>[2x]GAMNAQAEEFKKYLETNGIKPKQFHKKELIFNQWDPQEYCIFLYDGITKLTSISENGTIMNLQYYKGAFVIMSGFIDTETSVGYYNLEVISEQATAYVIKINELKELLSKNLTHFFYVFQTLQKQVSYSLAKFNDFSINGKLGSICGQLLILTYVYGKETPDGIKITLDNLTMQELGYSSGIAHSSAVSRIISKLKQEKVIVYKNSCFYVQNLDYLKRYAPKLDEWFYLACPATWGKLN

Expression of these L. monocytogenes virulence genes is controlled by positive regulatory factor A, PrfA. PrfA belongs to the cyclic AMP receptor protein-fumarate and nitrate reduction regulator (Crp-Fnr) family of bacterial transcription factors. Transcription factors of this family bind a wide range of ligands and are activated by allosteric communication between the ligand binding site and DNA-binding helix-turn-helix (HTH) motifs. Reduced glutathione (GSH), a low molecular weight thiol important for intracellular redox homeostasis, is thus far the only known allosteric activator of PrfA.

To verify and elucidate structural details of PrfA inhibition by IWP-2, we determined the crystal structure of the PrfA:IWP-2 complex at 2.0 Å resolution. The asymmetric unit of the PrfA:IWP-2 complex crystals contained one PrfA dimer composed of monomers A and B. Difference Fourier and Polder electron density maps unambiguously confirmed binding of IWP-2 to PrfA in monomer A, at the AI site, but not the BI site in monomer B. IWP-2 bound at the AI site with mostly hydrophobic interactions, as well as one direct hydrogen bond with the side chain of Gln146, and one water-mediated hydrogen with the side chains of Gln61, Tyr126 and Gln146. The ring-fused pyrimidone group of IWP-2 was positioned at site S1 in the vicinity of the aromatic side chains of residues Tyr126 and Phe67. The methyl-benzothiazole group of IWP-2 was directed towards, and pushed on, the first helix of the HTH motif. This resulted in a shift of the helix and folding into a structural conformation similar to that present in the GSH-activated PrfA structure. However, the binding of IWP-2 likely prevents the collapse of the N-terminal PrfA domain, a process otherwise necessary to line up the folded HTH motifs—one in each monomer—in positions compatible with palindromic DNA binding. As a result, in the IWP-2-bound PrfA structure, even though it is folded, the HTH motif has a position not compatible with DNA binding. In the PrfA monomer B, where no IWP-2 bound, the HTH motif was not folded. IWP-2 was 2.6-times more potent in inhibiting hly expression of L. monocytogenes in liquid culture compared to the recently described bicyclic 4-(1-naphthylmethyl)-2-pyridone PrfA inhibitor, KSK67 (15); IWP-2 IC50 = 0.026 μM versus KSK67 IC50 = 0.067 μM.> NGVPSTNVNTPAPNTGQSTAQNTN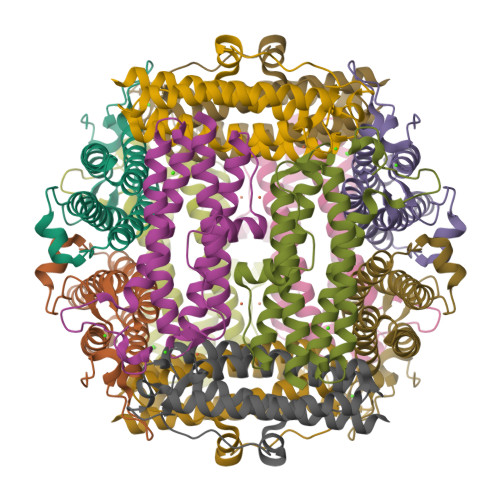TASPLPYNRATTLPAAGTEDLKKSVQALQNTLTELQALQLQTKQAHWNVSGTLWYTLHELLQDHYEGISKFADDVAERQLSVGASSDGRAITIVAASRLPEIPGGFLDDAQVIQFFTYQYETVGQRIHQRVGDVEKVDPTTANLLQEVEHIIEKYQWQMRAFLQNTPTDPNTGFDINNGKPVPLR>GSANLKNKTLVVTTILSNPYCMRKESAIPLSGNDQFEGYAVDLIHEISKSLGFNYKIQLVPDGSYGSLNKLTGEWNGM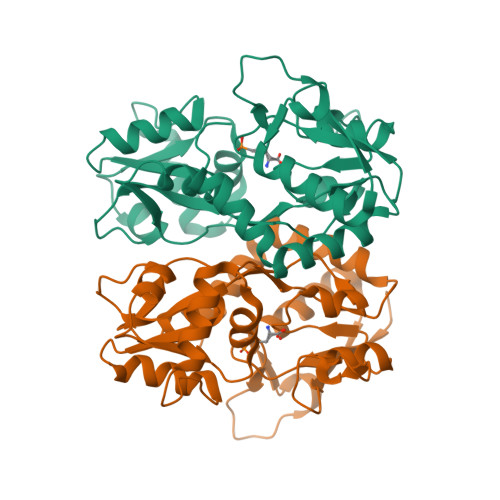IRELLEQRADLAIADLTITFEREQAVDFTTPFMNLGVSILYRKGTPIESAEDLAKQTRIKYGALKGGSTAAFFRDSKISTYQRMWSFMESARPSVFTASNGEGVERVAKGKGSYAFLMESTSIEYVTERNCELTQVGGMLDTKSYGIATPPNSPYRTAINSVILKLQEEGKLHILKTKWWKEKRGGGKCR[2x]> MNLLIDNWIPVRPRNGGKVQIINLQSLYCSRDQWRLSLPRDDMELAALALLVCIGQIIAPAKDDVEFRHRIMNPLTEDEFQQLIAPWIDMFYLNHAEHPFMQTKGVKANDVTPMEKLLAGVSGATNCAFVNQPGQGEALCGGCTAIALFNQANQAPGFGGGFKSGLRGGTPVTTFVRGIDLR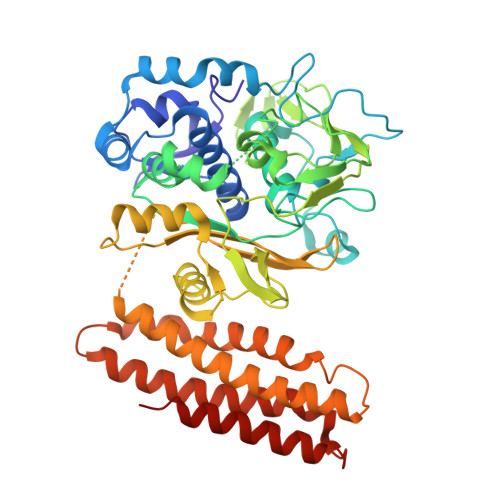STVLLNVLTLPRLQKQFPNESHTENQPTWIKPIKSNESIPASSIGFVRGLFWQPAHIELCDPIGIGKCSCCGQESNLRYTGFLKEKFTFTVNGLWPHPHSPCLVTVKKGEVEEKFLAFTTSAPSWTQISRVVVDKIIQNENGNRVAAVVNQFRNIAPQSPLELIMGGYRNNQASILERRHDVLMFNQGWQQYGNVINEIVTVGLGYKTALRKALYTFAEGFKNKDFKGAGVSVHETAERHFYRQSELLIPDVLANVNFSQADEVIADLRDKLHQLCEMLFNQSVAPYAHHPKLISTLALARATLYKHLRELKPQGGPSNG> RKPTALIILDGFGLREETYGNAVAQAKKPNFDGYWNKFPHTTLTACGEAVGLPEG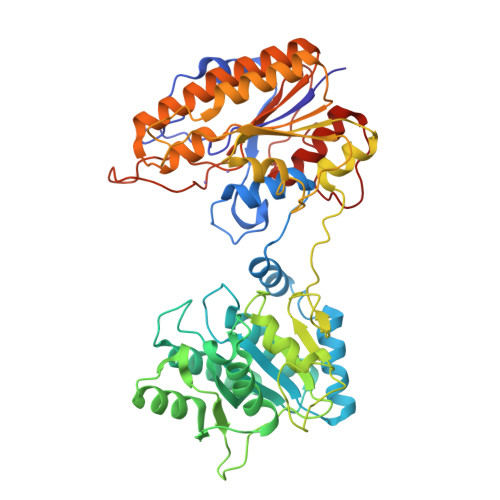QMGNSEVGHLNIGAGRIVYQSLTRVNVAIREGEFDKNETFQSAIKSVKEKGTALHLFGLLSDGGVHSHMNHMFALLRLAAKEGVEKVYIHAFLDGRDVGPKTAQSYIDATNEVIKETGVGQFATISGRYYSMDRDKRWDRVEKCYRAMVNGEGPTYKSAEECVEDSYANGIYDEFVLPSVIVNEDNTPVATINDDDAVIFYNFRPDRAIQIARVFTNGDFREFDRGEKVPHIPEFVCMTHFSETVDGYVAFKPMNLDNTLGEVVAQAGLKQLRIAETEKYPHVTFFFSGGREAEFPGEERILINSPKVATYDLKPEMSIYEVTDALVNEIENDKHDVIILNFANCDMVGHSGMMEPTIKAVEATDECLGKVVEAILAKDGVALITADHGNADEELTSEGEPMTAHTTNPVPFIVTKNDVELREDGILGDIAPTMLTLLGVEQPKEMTGKTIIK> MSQSNRELVVDFLSYKLSQKGYSWSQMAAVKQALREAGDEFELRYRRAFSDLTSQLHITPGTAYQSFEQVVNELFRDG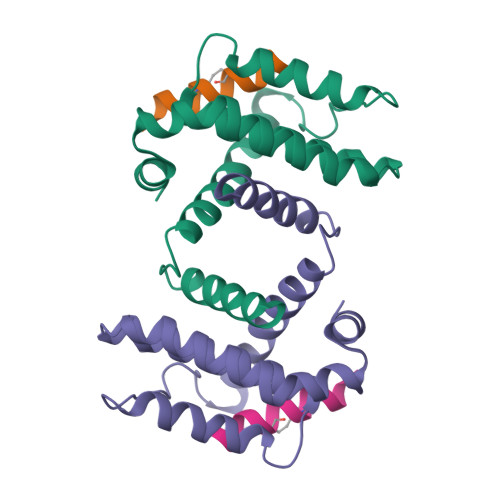VNWGRIVAFFSFGGALCVESVDKEMQVLVSRIAAWMATYLNDHLEPWIQENGGWDTFVELYGNNAAAESRKGQER;> XIWIAQELRLIGDLFNAYYARR>[4x]MDIKINDITLGNNSPFVLFGGINVLESLDSTLQTCAHYVEVTRKLGIPYIFKASFDKARSSIHSYRGVGLEEGLKIFEKVKAEFGIPVITDVHEPHQCQPVAEVCDVIQLPAFLARQTDLVVAMAKTGNVVNIKKPQFLSPSQMKNIVEKFHEAGNGKLILCERGSSFGYDNLVVDML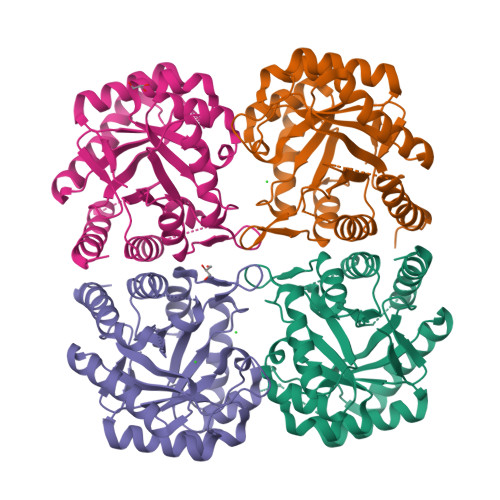GFGVMKQTCGNLPVIFDVTHSLQTRDAGSAASGGRRAQALDLALAGMATRLAGLFLESHPDPKLAKCDGPSALPLHLLEDFLIRIKALDDLIKSQPILTIE>[8x]GPLG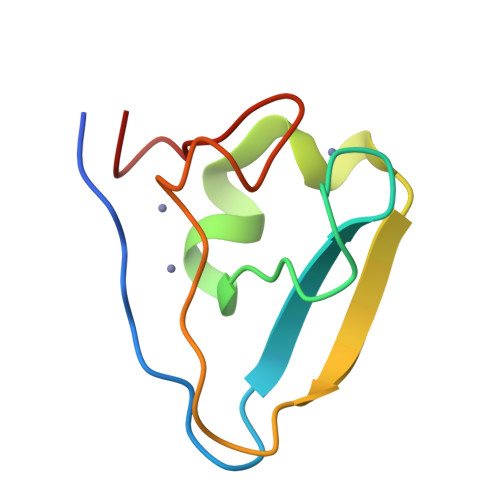SLCGRVFKVGEPTYSCRDCAVDPTCVLCMECFLGSIHRDHRYRMTTSGGGGFCDCGDTEAWKEGPYCQKHE>[4x]LGKFSQTCYNSAIQGSVLTSTCERTNGGYNTSSIDLNSVIENVDGSLKWQGSNFIETC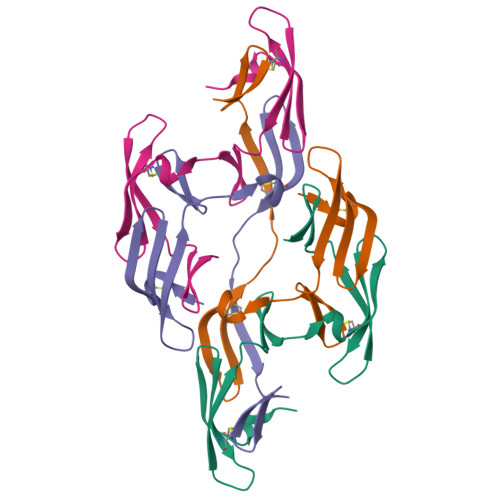RNTQLAGSSELAAECKTRAQQFVSTKINLDDHIANIDGTLKYE>[2x]MAIKRGADLIVEALEEYGTEQVVGFIGHTSHFVADAFSKSHLGKRVINPATELGGAWMVNGYNYVKDRSAAVGAWHCVGNLLLHAAMQEARTGRIPAVHIGLNSDGRLAGRSEAAQQVPWQSFTPIARSTQRVERLDKVGEAIHEAFRVAEGHPAGPAYVDIPFDLTADQIDDKALVPRGATRAKSVLHAPNEDVREAAAQLVAAKNPVILAGGGVARSGGSEALLKLAEMVGVP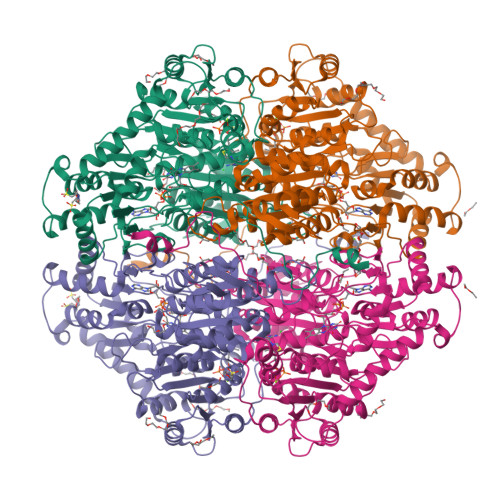VVTTSTGAGVFPETHALAMGSAGFCGWKSANDMMAAADFVLVLGSRLSDWGIAQGYITKMPKFVHVDTDPAVLGTFYFPLLSVVADAKTFMEQLIEVLPGTSGFKAVRYQERENFRQATEFRAAWDGWVREQESGDGMPASMFRAMAEVRKVQRPEDIIVTDIGNHTLPMFGGAILQRPRRLVTSMAEGILGCGFPMALGAQLAEPNSRVFLGTGDGALYYHFNEFRVAVEHKLPVITMVFTNESYGANWTLMNHQFGQNNWTEFMNPDWVGIAKAFGAYGESVRETGDIAGALQRAIDSGKPALIEIPVSKTQGLASDPVGGVGPNLLLKGREIPVDTGGSMYPGENLLHLKS>ALLITKKCINC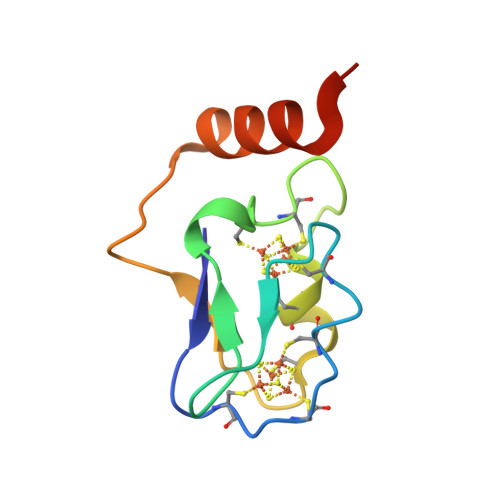DMCEPECPNEAISMGDHIYEINSDKCTECVGHYETPTCQKVCPIPNTIVKDPAHVETEEQLWDKFVLMHHADKI[3x]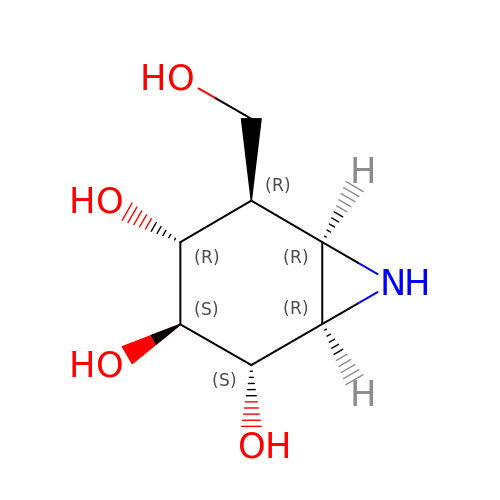(1~{R},2~{S},3~{S},4~{R},5~{R},6~{R})-5-(hydroxymethyl)-7-azabicyclo[4.1.0]heptane-2,3,4-triol | C7 H13 N O4 | GPIFFOGPRPKRHS-DRYVTRLFSA-N> ARRSVAARSSAPELWTPTSEVKLAVSSRNPHPPVVCQGPPPPNPLVIERFQGVVSQLFQQRIVR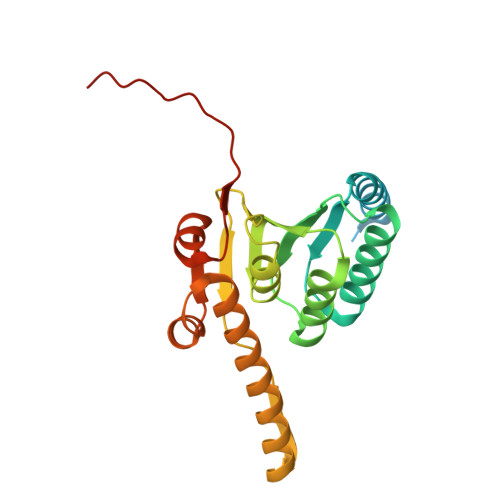LGGAVDDDMANLLVAQLLYLDSVDNKRDITMYVNSPGGSVTAGMAVFDTMRHIRPDVSTCCIGLAASMGAFILASGQAGKRYSLPNSRIMIHQPLGGAQGQATDIEIQANEILHHKLTLNGYLAQFTGQSMETITKDTDRDFFMSPQEAIEYGLVDAIISKPQMLQSREVALSS> GPISEFPVDFHYGVRVDVTLLSKIRRVNEHIKSATKTGVVQVHGSACTPTLSVLSSVGTAGVLGLRIKNALTPLVGHTEGSGDVSFSFRNTSVGSGFTHTRELFGANVLDAGIAFYRKGEACDTGAQPQFVRTTISYGDNLTSTVHKSVVDQKGILPFHDRMEAGGRTTRLLLCGKTGAFLLKWLRQQKTKEDQTVTVSVSETLSIVTFSLGGVSKIIDFKPETKPVSGWDGLKGKKSVDVGVVHTDALSRVSLESLIAALRLCKVPGWFTPGLIWHSNEILEVEGVPTGCQSGDVKLSVL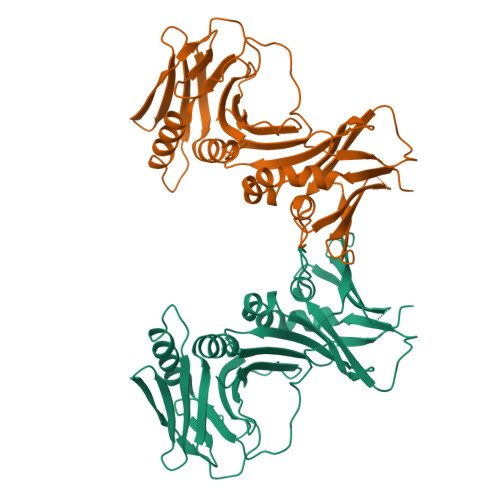LLEVNRSV>[2x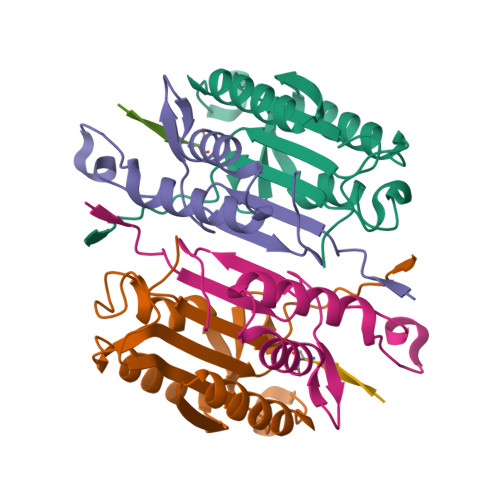]DNSYKMDYPEMGLCIIINNKNFHKSTGMTSRSGTDVDAANLRETFRNLKYEVRNKNDLTREEIVELMRDVSKEDHSKRSSFVCVLLSHGEEGIIFGTNGPVDLKKITNFFRGDRCRSLTGKPKLFIIQACRGTELDCGIET;>CHKIPVEADFLYAYSTAPGYYSWRNSKDGSWFIQSLCAMLKQYADKLEFMHILTRVNRKVATEFESFSFDATFHAKKQIPCIVSMLTKELYFYHH[2x];>[2x]XITAKD>[2x]MKIGCHGLVWTGHFDAEGIRYSVQKTREAGFDLVEFPLMDPFSFDVQTAKSALAEHGLAASASLGLSDATDVSSEDPAVVKAGEEL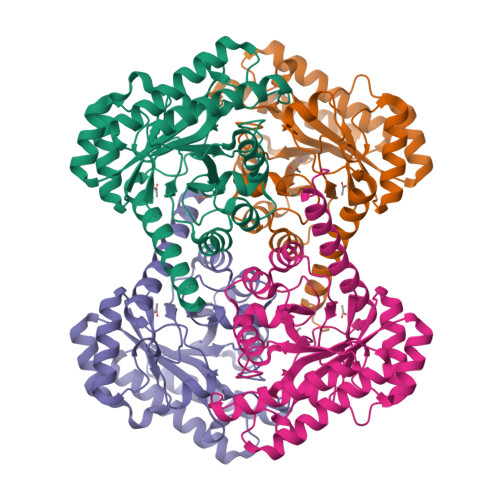LNRAVDVLAELGATDFCGVIYSAMKKYMEPATAAGLANSKAAVGRVADRASDLGINVSLEVVNRYETNVLNTGRQALAYLEELNRPNLGIHLDTYHMNIEESDMFSPILDTAEALRYVHIGESHRGYLGTGSVDFDTFFKALGRIGYDGPVVFESFSSSVVAPDLSRMLGIWRNLWADNEELGAHANAFIRDKLTAIKTIELHRSHHHHHH4-(2-{[(2-aminoquinolin-7-yl)methyl]amino}ethyl)-2-chlorobenzonitrile | C19 H17 Cl N4 | 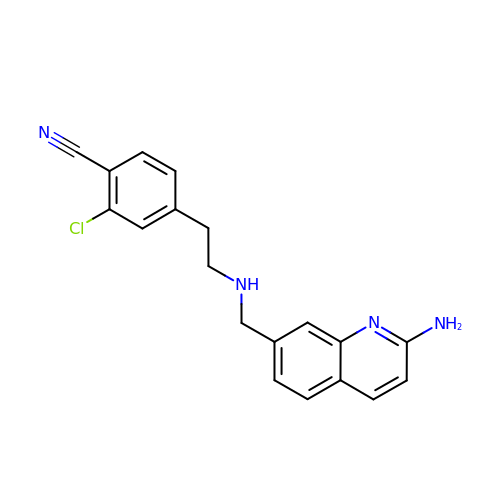KZMLSFIKJMMRRD-UHFFFAOYSA-N>[2x]ASKPQPIAAANWKCNGSESLLVPLIETLNAATFDHDVQCVVAPTFLHIPMTKARLTNPKFQIAAQNAITRSGAFTGEVSLQILKDYGISWVVLGHSERRLYYGETNEIVAEKVAQACAAGFHVIVCVGETNEEREAGRTAAVVLTQLAAVAQKLSKEAWSRVVIAYEPVWAIGTGKVATPQQAQEVHELLRRWVRSKLGTDIAAQLRILYGGSVTAKNARTLYQMRDINGFLVGGASLKPEFVEIIEATK

Triosephosphate isomerase (TIM) is a ubiquitous enzyme that catalyzes the interconversion between glyceraldehyde 3-phosphate and dihydroxyacetone phosphate. TIM belongs to the family of α-β barrels proteins, in which 8 central β strands are surrounded by 8 α helices; the strands and helices are joined by loops. A peculiarity of TIM is that only in its dimeric form the enzyme exhibits high catalytic rates, albeit each monomer has its own catalytic residues. DTDA is a powerful inhibitor of the activity of TIM from T. cruzi.

On the other hand we were able to obtain crystals of the complex by soaking crystals of TcTIM with 1 mM DTDA. The RMS deviation of the Cα traces of native TcTIM and the DTDA treated enzymes was 0.39 Å. The data also showed that in the position of Cys118, which is far from the interface, the two monomers exhibited electron densities that fitted well with a structure in which the sulfur of Cys118 was covalently linked through a disulfide bond to a thioaniline moiety.Thus, in TcTIM crystals, DTDA was able to derivatize Cys118; however, as shown by the data on the Cys118Val mutant, the inhibition of activity by the compound does not depend on the perturbation of Cys118. Accordingly, and in regard to the inhibition of activity of TcTIM by DTDA, it is relevant that the enzyme soaked with DTDA exhibited significant and rather unique alterations in its dimer interface. One of the most notable was that although loop3 of monomer B exhibited a conformation almost identical to that in native TcTIM, loop3 of monomer A acquired a markedly different conformation. In monomer A of the DTDA treated enzyme, residues 66 to 70 and residues 77 to 79 superpose quite well with those of the “normal” loop, however, the region formed by residues 71 to 76 exhibited a significant displacement with a hinge at the level of Thr70 and Thr76. The change in conformation of loop3 of monomer A was accompanied by alterations in the contacts that it establishes with residues of monomer B. In native TcTIM, the side chain of Cys15 of the two subunits is well defined, and their N and O atoms are respectively, hydrogen bonded to the O and N atoms of Gly73 of the adjacent subunit. In the DTDA treated enzyme, these H-bonds are missing. This was consequence of an increase in the distance between Gly73 of monomer A and Cys15 of the other subunit; in the treated enzyme, the distances between N and O atoms of Gly73 and the O and N atoms of Cys15 were 7.9 and 9.2 Å, respectively. Therefore, it is likely that in the crystal, an intermediate of the overall conformational changes induced by DTDA was trapped.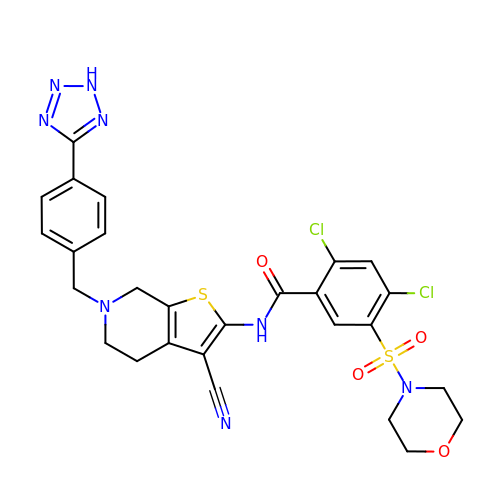N-(6-(4-(2h-tetrazol-5-yl)benzyl)-3-cyano-4,5,6,7-tetrahydrothieno[2,3-c]pyridin-2-yl)-2,4-dichloro-5-(morpholinosulfonyl)benzamide | C27 H24 Cl2 N8 O4 S2 | KXJHJZRFLLSTJD-UHFFFAOYSA-N> IQAVIAEQLNVDAAQVTPEAEFVKDLGADSLDVVELIMALEEKFGIEIPDEQAEKIVNVGDVV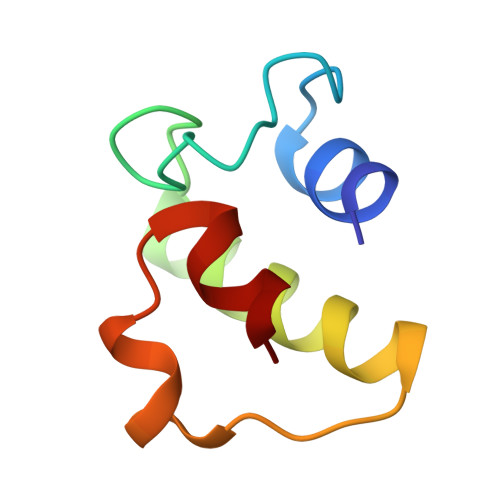KY> MNHKVHHHHHHIEGAAMNEFARKKRALEHSRRINAGDLDAIIDLYAPDAVLEDPVGLPPVTGHDALRAHYEPLLAAHLREEAAEPVAGQDATHALIQISSVMDYLPVGPLYAERGWLKAPDAPGTARIHRTAMLVIRMDASGLIRHLKSYWGTSDLSGGSGPAPDEAARKQMAVDYAERINAGDIEGVLDLFTDDIVFEDPVG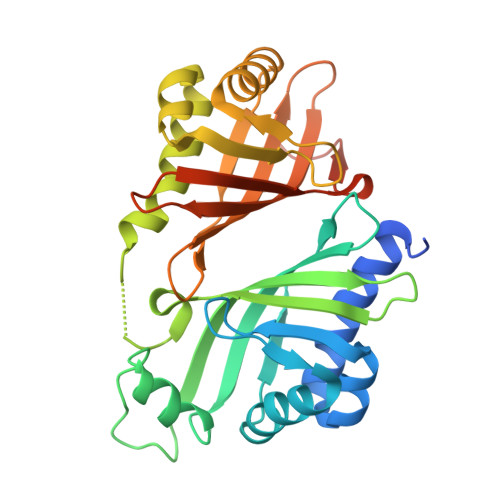RPPMVGKDDLRRHLELAVSCGTHEVPDPPMTSMDDRFVVTPTTVTVQRPRPMTFRIVGIVELDEHGLGRRVQAFWGVTDVTMDDRVQAFWGVTDVTMDD>[6x]MTSAEMTSPNNNSEHQAIAKMRTMIEGFDDISHGGLPIGRSTLVSGTSGTGKTLFSIQFLYNGIIEFDEPGVFVTFEETPQDIIKNARSFGWDLAKLVDEGKLFILDASPDPEGQEVVGGFDLSALIERINYAIQKYRARRVSIDSVTSVFQQYDASSVVRRELFRLVARLKQIGATTVMTTERIEEYGPIARYGVEEFVSDNVVILRNVLEGERRRRTLEILKLRGTSHMKGEYPFTITDHGINIFPLGAMRLTQRSSNVRVSSGVVRLDEMCGGGFFKDSIILATGATGTGKTLLVSRFVENACANKERAILFAYEESRAQLLRNAYSWGMDFEEMERQNLLKIVCAYPESAGLEDHLQIIKSEINDFKPARIAIDSLSALARGVSNNAFRQFVIGVTGYAKQEEITGLFTNTSDQFMGAHSITDSHIEEITDTIILLQYVEIRGEMSRAINVFKMRGSWHDKAIREFMISDK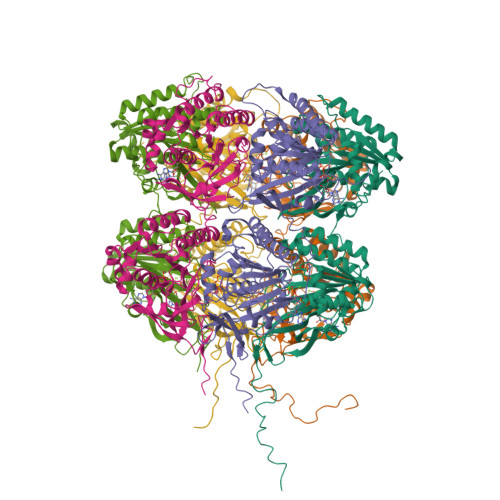GPDIKDSFRNFERIISGSPTRITVDEKSELSRIVRGVQEKGPESHHHHHH>MKIGSGEKLLFIGDSITDCGRARPEGEGSFGALGTGYVAYVVGLLQAVYPELGIRVVNKGISGNTVRDLKARWEEDVIAQKPDWVSIMIGINDVWRQYDLPFMKEKHVYLDEYEATLRSLVLETKPLV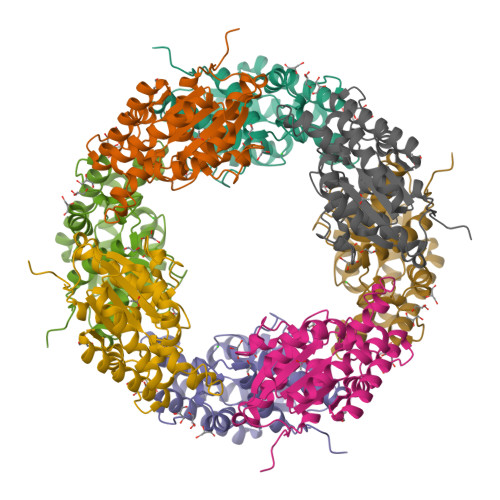KGIILMTPFYIEGNEQDPMRRTMDQYGRVVKQIAEETNSLFVDTQAAFNEVLKTLYPAALAIDRVHPSVAGHMILARAFLREIGFEWVRSR[2x]>EQDIYLPIANVARIMKNAIPQTGKIAKDAKECVQECVSEFISFITSEASERCHQEKRKTINGEDILFAMSTLGFDSYVEPLKLYLQKFR[2x];>QELPLARIKKIMKLDEDVKMISAEAPVLFAKAAQIFITELTLRAWIHTEDNKRRTLQRNDIAMAITKFDQFDFLIDIVPR[2x]

The transcription factor (TF) NF-Y is a nuclear protein that binds the CCAAT sequence in promoters with a very high specificity. NF-Y is a heterotrimer formed by evolutionarily conserved subunits: NF-YA, NF-YB, and NF-YC. NF-YB and NF-YC form a heterodimer via interacting histone fold domains (HFDs), while NF-YA provides DNA sequence-specificity to the trimer. The NF-YA subunit, once associated to the HFD dimer with its A1 α-helix, recognizes and binds the CCAAT nucleotides via its A2 α-helix and the following Gly-loop, inserting in the minor groove of DNA.

In this study, we demonstrated that suramin, a polysulfonated naphthylamine derivative of urea, inhibits the DNA interaction of NF-Y with the CCAAT box by binding the HFD subunits, either as isolated heterodimers or in the complete trimer. The NF-Yd–suramin co-crystals belonged to space group P212121 and diffracted to 2.7 Å resolution. The refinement converged to an Rfactor value of 22.2% (Rfree = 27.4%), with a final model composed of two NF-Yd protomers (identified with A/B, and C/D chains for NF-YB/NF-YC, respectively), one suramin molecule, one glycerol, one citrate, and 47 water molecules in the asymmetric unit. The suramin molecule adopts an elongated conformation in the (NF-Yd)2–suramin complex, and binds at the interface between two NF-Yd protomers, in an almost symmetric manner. Within the HFD heterodimer, NF-YC is the subunit that provides the majority of the suramin-interacting residues: located at the first turn of helix α1 and in the L1 region, they are mostly apolar and generate the homodimeric cleft where suramin symmetrically fits. Additionally, the C-terminus of the NF-YB subunit, in particular Arg140, provides an additional electrostatic interaction to stabilize a second suramin sulfonic acid group. In particular, the NF-YB Phe139 side chain rotates by about 90° to accommodate the two benzene rings attached to the urea moiety of the ligand. In the (NF-Yd)2–suramin complex, the ligand is located close to the DNA binding region of NF-Y, contacting NF-YC L1 and α1 and NF-YB αC, which are responsible for more than 40% of the contacts between the HFD NF-Yd and the phosphate backbone of the NF-Y-bound DNA. Furthermore, two sulfonic acid groups that decorate the suramin naphthalene moiety, in particular the one salt-bridged to the NZ atoms of NF-YC Lys49 and Lys53, match well with the position of two DNA phosphate groups, corresponding to position −21 and −20 in the complementary strand of the CCAAT box in the DNA/NF-Y complex. Furthermore, the suramin-induced homodimerization of the HFD heterodimers sterically precludes binding of about 10 bp present in the NF-Y/DNA complex.>[2x]MHHHHHHGKNHAGSPGCEESAAGKEKLPKMRLPTRSDMICGYACLKGTAAMRNTKRGSWYIEALAQVFSERACDMHVADMLVKVNALIKD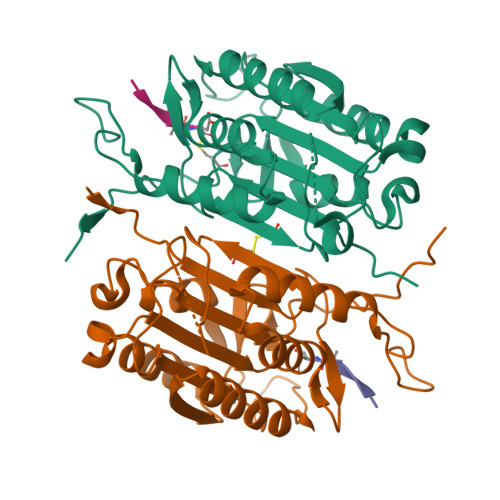REGYAPGTEFHRCKEMSEYCSTLCRHLYLFPGGGVKPCTPEFYQTHFQLAYRLQSRPRGLALVLSNVHFTGEKELEFRSGGDVDHSTLVTLFKLLGYDVHVLCDQTAQEMQEKLQNFAQLPAHRVTDSCIVALLSHGVEGAIYGVDGKLLQLQEVFQLFDNANCPSLQNKPKMFFIQACRGDETDRGVDQQD;>XVDVAD[2x]> MGSSHHHHHHENLYFQSNAAIASEFSSLPSYAAFATAQEAYEQAVANGDSEVVLKKLKKSLNVAKSEFDRDAAMQRKLEKMADQAMTQMYKQARSEDKRAKVTSAMQTMLFTMLRKLDND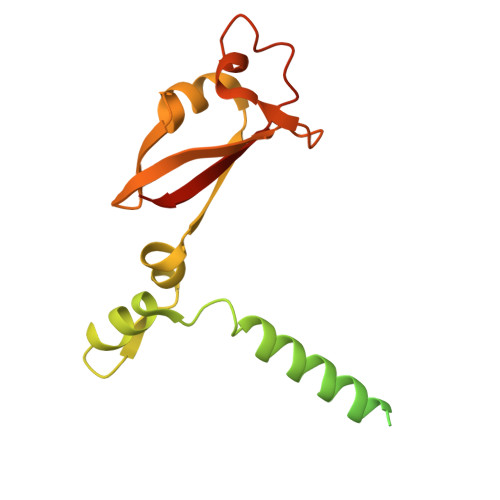ALNNIINNARDGCVPLNIIPLTTAAKLMVVIPDYNTYKNTCDGTTFTYASALWEIQQVVDADSKIVQLSEISMDNSPNLAWPLIVTALRANSAVKLQ The ferrous iron and 2-oxoglutarate (2OG)-dependent HIF prolyl hydroxylases (PHDs/EGLNs) catalyse trans-4-prolyl hydroxylations on HIFα subunits, thus promoting their binding to the von Hippel–Lindau protein (VHL), a targeting component of a ubiquitin E3 ligase, and signalling for HIFα degradation under normoxic conditions. The PHD-catalysed hydroxylations of HIF-1α/HIF-2α in higher animals occur in amino- and carboxy-terminal oxygen-dependent degradation domains (NODD and CODD). The three human PHDs exhibit different NODD/CODD selectivities, with PHD3 being substantially more selective for CODD than PHD1/2 (refs 16). Biophysical analyses employing crystallography and NMR reveal that the molecular basis of PHD isoform and variant selectivity involves enzyme–substrate interactions involving β2/β3 loop residues (that bind the LXXLAP motif) and helices α3 and α4, regions which display sequence variations between the PHD isoforms.

A PHD2 R396T variant, present in breast carcinoma, and an R396A variant efficiently hydroxylate NODD, but both manifest loss of CODD activity. Structures of the P317R, R371H and R396T variants with a clinically used inhibitor628 reveal similar overall folds to wt PHD2, that is, a modified double-stranded-β-helix (DSBH) core (β-strands I–VIII), supporting 2OG and His-X-Asp…His-mediated Fe(II) binding. The structures suggested that these variants probably manifest altered substrate binding, but do not explain how their differing NODD/CODD selectivities arise. Comparison of the structures rationalizes the selectivities of the clinically observed P317R, R371H and R396T variants. In the PHD2.CODD structure, Arg396PHD2 (α4) is positioned to salt bridge with Asp571CODD; analysis of the ODD structures leads to the prediction that the R396T and R396A substitutions disrupt their interaction with Asp571CODD, but will not directly have an impact on NODD binding. Indeed, structures of R396T with/without NODD indicate how R396T substitution is tolerated for NODD binding. In the case of R396T (which does not hydroxylate CODD efficiently, 2b), both FG2216 and FG4592 manifest NODD displacement less than wt PHD2.

> GSHMASPNGQTKPLPALKLALEYIVPCMNKHGICVVDDFLGKETGQQIGDEVRALHDTGKFTDGQLVSQKSDSSKDIRGDKITWIEGKEPGCETIGLLMSSMDDLIRHCNGKLGSYKINGRTKAMVACYPGNGTGYVRHVDNPNGDGRCVTCIYYLNKDWDAKVSGGILRIFPEGKAQFADIEPKFDRLLFFWSDRRNPHEVQPAYATRYAITVWYFDADETARAKVKYLTGEKGVRVELNKPSDSVGKDVF> MERYENLFAQLNDRREGAFVPFVTLGDPGIEQSLKIIDTLIDAGADALELGVPFSDPLADGPTIQNANLRAFAAGVTPAQCFEMLALIREKHPTIPIGLLMYANLVFNNGIDAFYARCEQVGVDSVLVADVPVEESAPFRQAALRHNIAPIFICPPNAD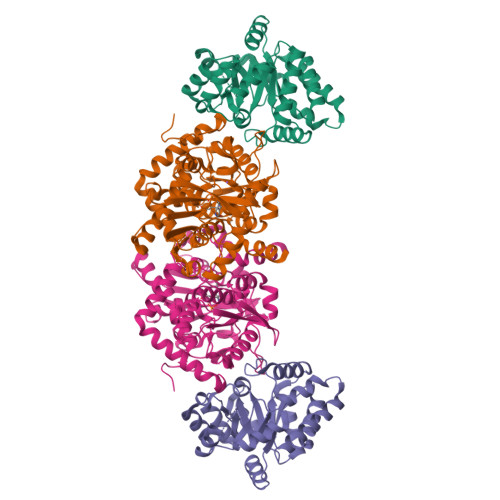DDLLRQVASYGRGYTYLLSRSGVVGAENRGALPLHHLIEKLKEYHAAPALQGFGISSPEQVSAAVRAGAAGAISGSAIVKIIEKNLASPKQMLAELRSFVSAMKAASRA;> MTTLLNPYFGEFGGMYVPQILMPALNQLEEAFVSAQKDPEFQAQFADLLKNYAGRPTALTKCQNITAGTRTTLYLKREDLLHGGAHKTNQVLGQALLAKRMGKSEIIAETGAGQHGVASALASALLGLKCRIYMGAKDVERQSPNVFRMRLMGAEVIPVHSGSATLKDACNEALRDWSGSYETAHYMLGTAAGPHPYPTIVREFQRMIGEETKAQILDKEGRLPDAVIACVGGGSNAIGMFADFINDTSVGLIGVEPGGHGIETGEHGAPLKHGRVGIYFGMKAPMMQTADGQIEESYSISAGLDFPSVGPQHAYLNSIGRADYVSITDDEALEAFKTLCRHEGIIPALESSHALAHALKMMREQPEKEQLLVVNLSGRGDKDIFTVHDILKARGEI> MIRYKGFILFL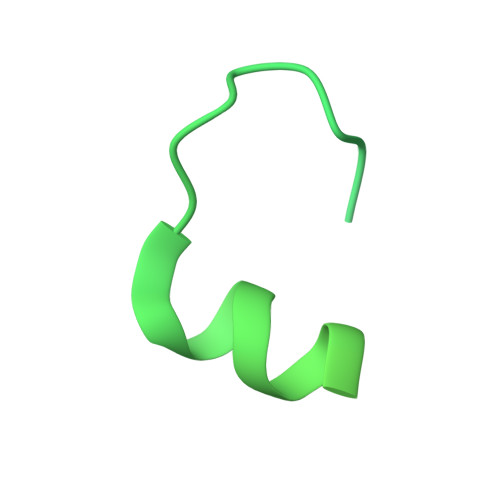LLMLIGCEQREELISNLSQRQANEIISVLERHNITARKVDGGKQGISVQVEKGTFASAVDLMRMYDLPNPERVDISQMFPTDSLVSSPRAEKARLYSAIEQRLEQSLVSIGGVISAKIHVSYDLEEKNISSKPMHISVIAIYDSPKESELLVSNIKRFLKNTFSDVKYENISVILTPKEEYVYTNVQPVKEVKSEFLTNEVIYLFLGMAVLVVILLVWAFKTGWFKRNKI> MVESNDII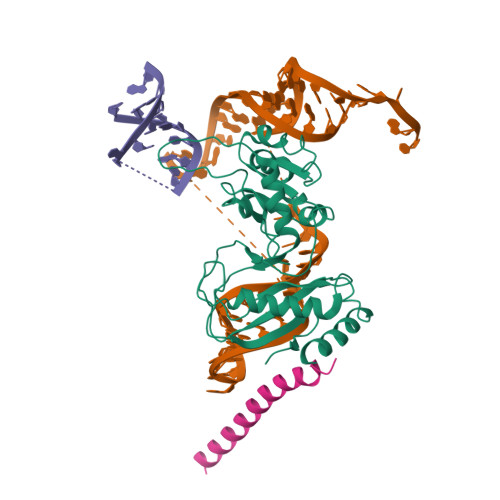KSGLAEKALKALILQCEENPSLKNDKDIHIIINTGKKMGINRDNIPRIIPLTKYKLFKPRDLNILLITKDPSALYRETLTKDEHTSELFKEIISVKNLRRRFKGSKLTQLYKDFDLVVADYRVHHLLPEVLGSRFYHGSKKLPYMIRMSKEVKLKRQQMVEKCDPIYVRAQLRSICKNTSYIPNNDNCLSVRVGYIQKHSIPEILQNIQDTINFLTDKSKRPQGGVIKGGIISIFVKTSNSTSLPIYQFSEARENQKNEDLSDIKL SARS-CoV-2 encodes four structural proteins incorporated into virions, spike (S), envelope (E), nucleocapsid (N), and membrane (M). M plays an essential role in viral assembly by organizing other structural proteins through physical interactions and directing them to sites of viral budding. As the most abundant protein in the viral envelope and a target of patient antibodies, M is a compelling target for vaccines and therapeutics. M forms a 50 kDa homodimer that is structurally related to the SARS-CoV-2 ORF3a viroporin, suggesting a shared ancestral origin.

We reconstituted homodimeric SARS-CoV-2 M in nanodiscs made from the scaffold protein MSP1E3D1 and lipids (DOPE:POPC:POPS in a 2:1:1 ratio) and determined its structure by cryo-EM. The majority of M (189 of 222 amino acids per subunit) was de novo modeled in the cryo-EM map. Each subunit contains an extracellular or lumenal N-terminus, three transmembrane helices (amino acids 17–36, 43–71, and 79–105) connected by short linkers, and a β-strand rich C-terminal cytosolic domain. The two subunits assemble along their long axis, with TM1 from one protomer forming extensive interactions with the TM2-TM3 unit of the second protomer. The inner sheets from each protomer interact through a large (~690 Å2 buried surface area per chain) and complementary interface with residues L138, V139, V143, L145, F193, A195 contributing to a hydrophobic core surrounded by additional polar interactions. Second, the M pocket is completely sealed by protein to the surrounding membrane and cytoplasm; no openings large enough for water passage are observed connecting the pocket and protein exterior. In M, the gap between subunits is confined to the region between cytosolic domains because transmembrane helices from opposing subunits form tight interactions across the entire lipid bilayer. The cytosolic domain of M is strikingly electropositive across nearly the entire exposed surface. Taken together, these data suggest that M adopts a stable structure with minimal dynamic rearrangements on the microsecond timescale, at physiological temperature, and in the absence of additional binding proteins. Our data suggests that M in a simple lipid mixture predominantly adopts the short form.

>MADSNGTITVEELKKLLEQWNLVIGFLFLTWICLLQFAYANRNRFLYIIKLIFLWLLWPVTLACFVLAAVYRINWITGGIAIAMACLVGLMWLSYFIASFRLFARTRSMWSFNPETNILLNVPLHGTILTRPLLESELVIGAVILRGHLRIAGHHLGRCDIKDLPKEITVATSRTLSYYKLGASQRVAGDSGFAAYSRYRIGNYKLNTDHSSSSDNIALLVQSNSLEVLFQ[2x]> SHMANKREPAPGWPIVSGEYVVGNPESCVGVVTLGSHGLEQACIDAGAAIAGPCHTENLGIEKVVANYISNPNIRFMILCGSEVQGHITGQCFKALWENGIGDDGGIIGAKGAIPFLENVNKEAVERFRRQIVEVVDLIDCEDIGKITQAIKECLSKDPGAIDEDPFIIELE;> GSHMANKREPAPGWPIVSGEYVVGNPESCVGVVTLGSHGLEQACIDAGAAIA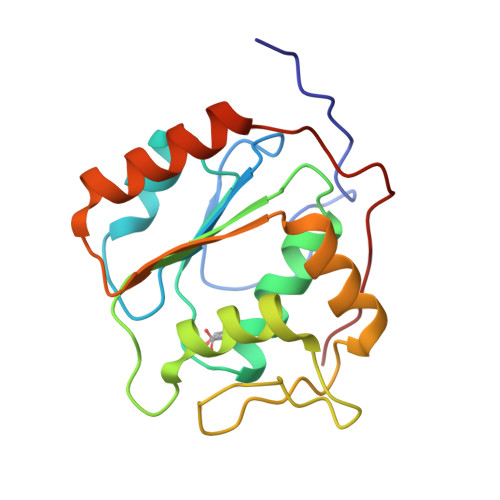GPCHTENLGIEKVVANYISNPNIRFMILCGSEVQGHITGQCFKALWENGIGDDGGIIGAKGAIPFLENVNKEAVERFRRQIVEVVDLIDCEDIGKITQAIKECLSKDPGAIDEDPFIIELE>[2x]MAALMTPGTGAPPAPGDFSGEGSQGLPDPSPEPKQLPELIRMKRDGGRLSEADIRGFVAAVVNGSAQGAQIGAMLMAIRLRGMDLEETSVLTQALAQSGQQLEWPEAWRQQLVDKHSTGGVGDKVSLVLAPALAACGCKVPMISGRGLGHTGGTLDKLESIPGFNVIQSPEQMQVLLDQAGCCIVGQSEQLVPADGILYAARDVTATVDSLPLITASILSKKLVEGLSALVVDVKF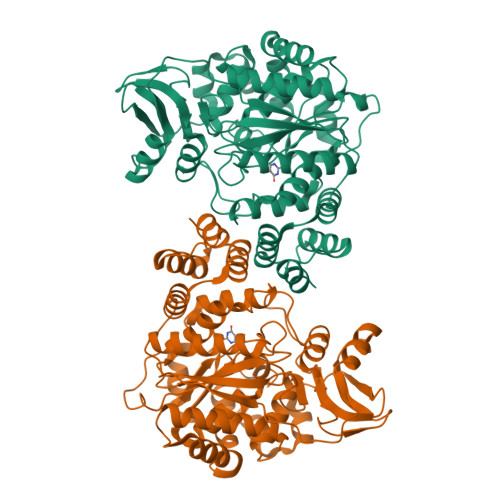GGAAVFPNQEQARELAKTLVGVGASLGLRVAAALTAMDKPLGRCVGHALEVEEALLCMDGAGPPDLRDLVTTLGGALLWLSGHAGTQAQGAARVAAALDDGSALGRFERMLAAQGVDPGLARALCSGSPAERRQLLPRAREQEELLAPADGTVELVRALPLALVLHELGAGRSRAGEPLRLGVGAELLVDVGQRLRRGTPWLRVHRDGPALSGPQSRALQEALVLSDRAPFAAPSPFAELVLPPQQ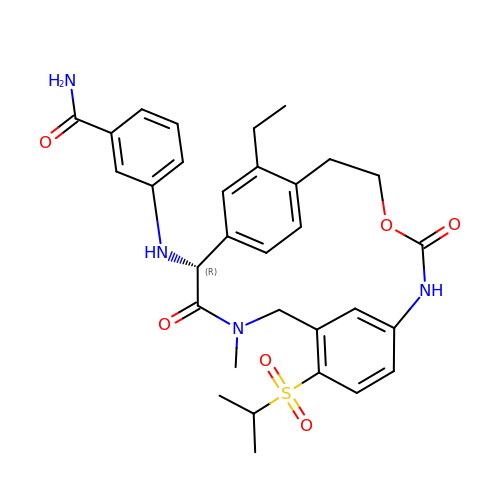3-{[(2R)-17-ethyl-4-methyl-3,12-dioxo-7-[(propan-2-yl)sulfonyl]-13-oxa-4,11-diazatricyclo[14.2.2.1~6,10~]henicosa-1(18),6(21),7,9,16,19-hexaen-2-yl]amino}benzamide | C31 H36 N4 O6 S | KZSYSYPLRUUKEU-MUUNZHRXSA-N>GESKKDRNTETNTETKSVPEEMEASKYVGQGFQPPAEKDAIEFSKKHKDKIAKRGEQFFMDNFGLKVKATNVVGSGDGVEVFVHCDDHDIVFNASIPFDKSIIESDSS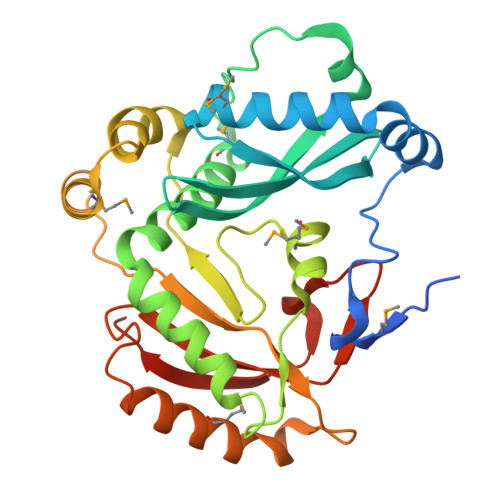LRSEDKGDDMSTLVGTVLSGFEYRAHKEELDNLTEVLKEYKSKYKYTGYTENAIMKTQNSGFRNEYYYLTAIPYTLDEYKRYFQPLIKEDDKSFRDGMRNSKKQLKDKSRPYVVTTLFSTKDNFTKDNTIDEMIDFSEVLKKKKNIPHDLNVSLQISNKYINTKRPNYSKKEVIEVGVFNHEKANTND[2x]>AQVINTFDGVADYLQTYHKLPDNYITKSEAQALGWVASKGNLADVAPGKSIGGDIFSNREGKLPGKSGRTWREADINYTSGFRNSDRILYSSDWLIYATTDHYQTFTKIR[2x];>MKKAVINGEQIRSIS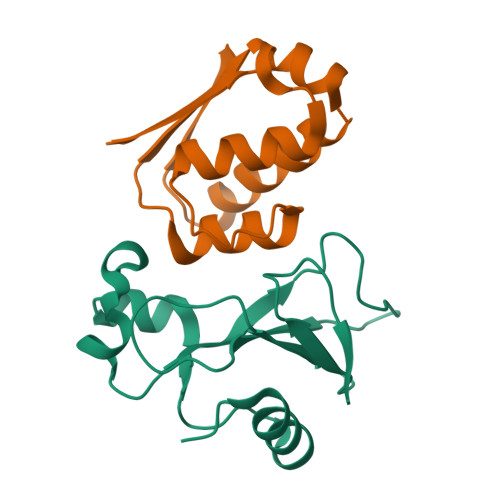DLHQTLKKELALPEYYGENLDALWAALTGWVEYPLVLEWRQFEQSKQLTENGAESVLQVFREAKAEGADITIILS[2x]> AVNGKGMNPDYKAYLMAPLKKIPEVTNWETFENDLRWAKQNGFYAITVDFWWGDMEKNGDQQFDFSYAQRFAQSVKNAGMKMIPIISTHQCGGNVGDDCNVPIPSWVWNQKSDDSLYFKSETGTVNKETLNPLASDVIRKEYGELYTAFAAAMKPYKDVIAKIYLSGGPAGELRYPSYT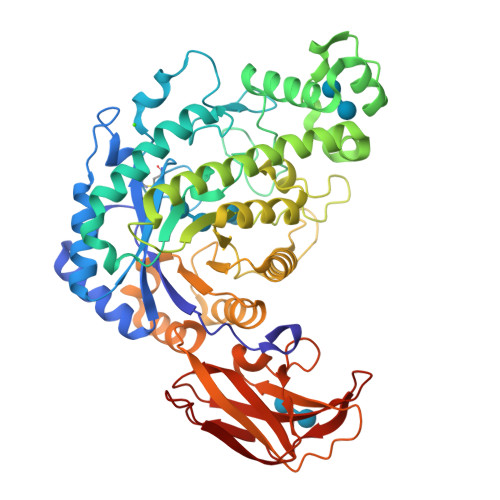TSDGTGYPSRGKFQAYTEFAKSKFRLWVLNKYGSLNEVNKAWGTKLISELAILPPSDGEQFLMNGYLSMYGKDYLEWYQGILENHTKLIGELAHNAFDTTFQVPIGAKIAGVHWQYNNPTIPHGAEKPAGYNDYSHLLDAFKSAKLDVTFTCLEMTDKGSYPEYSMPKTLVQNIATLANEKGIVLNGENALSIGNEEEYKRVAEMAFNYNFAGFTLLRYQDVMYNNSLMGKFKDLLGVTPVMQTIVVKNVPTTIGDTVYITGNRAELGSWDTKQYPIQLYYDSHSNDWRGNVVLPAERNIEFKAFIKSKDGTVKSWQTIQQSWNPVPLKTTSHTSSW> GDSAPLNEAMAVLQHHDAVSGTSRQHVANDYARQLSEGWRPCEVLMSNALAHLSGLKEDFAFCRKLNISICPLTQTAERFQVIVYNPLGRKVDWMVRLPVSKHVYLVKDPGGKIVPSDVVTIPSSDSQE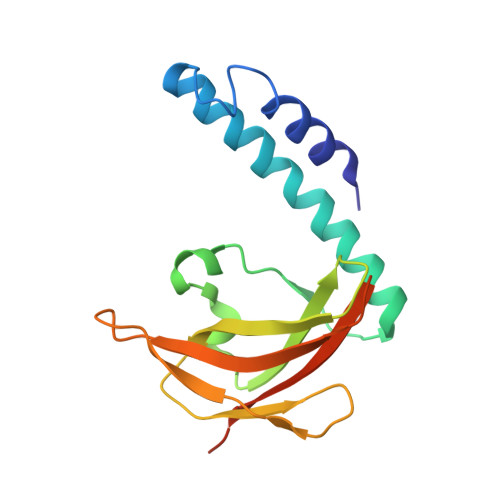LLFSALVPAVGFSIYSVSQMPNQRPQKSWS> MSAIKRSLNVGVVGMGNMGVPIARNLGFKARSAMYLQIHSRALSKAKRVCDDLSVDGATC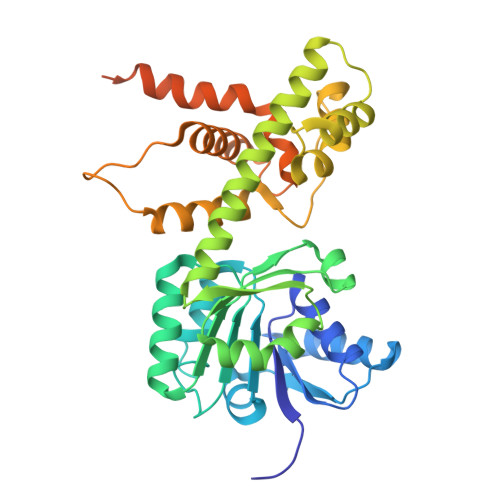AMRIHDRYSTMTKWCDVIVLALADVKASRHALLEDNESLIMNARKGQIIVDHTTVDAETSRECAHEAARRGAYFLDAPMSGSPRACFNGQLLLMVGGDAETFQKMLPIFHMYADNVFHMGESGSGTAAKMISQALVASHNAAAAEALSMAHALGIEDQSKLVQVLDASWGSSTMLRRNAPLLQDLIRNPDKTPPTSAVSVDRLLSDLAHLDASLPKRGGEDEPFPVFDAALRSLAAASDAGMGDRDLASVVHYIEAGEAELRNRTHVPLGGEHLTGRTAATAANSSVNETPSTVNGSSEVPNEFGVEDFY One such enzyme is 2-hydroxyacyl-CoA lyase/synthase (HACL/S), which catalyzes the reversible cleavage of 2-hydroxyacyl-CoA (2hcCoA) into formyl-CoA (fCoA) and an aldehyde or ketone. Originally identified in the mammalian α-oxidation pathway of 3-methyl-branched fatty acids, HACL/S has demonstrated remarkable catalytic reversibility, as it is capable of condensing fCoA with various substrates covering a wide range of aldehydes and ketones with different carbon chain lengths. All the enzymes are tetramers, specifically dimers of dimers (α2), where α2 dimer represents a catalytical unit. The three domains have specific functions: the N-terminal domain binds the pyrimidine of ThDP (PYR), the middle domain has a regulatory function (R) and binds ADP, and the C-terminal domain binds the pyrophosphoryl group (PP) of ThDP.

Of particular interest here are the structures of ApbHACL/S with fCoA and D-/L-lCoA. In the structure of ApbHACL/S incubated with fCoA, we trapped a covalent intermediate corresponding to ThDP-hmCoA. This adduct is a product of deprotonated ThDP reacting with fCoA. In these two structures ApbHACACL/S-CoA and ApbHACL/S-fCoA, the distances between C2 of ThDP and C1 of hmCoA are significantly longer than a regular C–C bond (1.54 Å) with 1.8 and 1.9 Å, respectively. Additionally, the C1-O distance in ApbHACL/S-CoA is 1.4 Å which is close to that of a regular hydroxymethyl but 2.0 Å for the same distance in ApbHACL/S-fCoA is much elongated. This suggests that these two intermediates found in these structures represent slightly different reaction states. Similarly, hCoA is partly ordered in the structure of TbHACL/S. Remarkably, in the structure with fCoA there is an intermediate trapped where there is a covalent bond between C2 of ThDP and carbon of hydroxymethyl moiety that is still attached to the sulfur atom of CoA. This seemingly corresponds to the intermediary α−carbanion state with ThDP covalently attached to hmCoA with an elongated C2-C bond distance. Moreover, ApbHACL/S shows the lowest KM (0.41 mM) toward acetaldehyde, which could contribute to successful crystallization with formyl-CoA and acetaldehyde, in addition to lactyl-CoA.

>[4x]SNAMAKSEGKVNGATLMARALQQQGVQYMFGIVGFPVIPIAIAAQREGITYIGMRNEQSASYAAQAASYLTGRPQACLVVSGPGVVHALAGLANAQVNCWPMLLIGGASAIEQNGMGAFQEERQVLLASPLCKYAHQVERPERIPYYVEQAVRSALFGRPGAAYLDMPDDVILGEVEEAAVRPAATVGEPPRSLAPQENIEAALDALQSAKRPLVIVGKGMAWSRAENEVRQFIERTRLPFLATPMGKGVMPDDHPLSVGGARSHALQEADLVFLLGARFNWILHFGLPPRYSKDVRVIQLDLSAEEIGNNRQAEVALVGDGKAIVGQLNQALSSRQWFYPAETPWREAIAAKIAGNQAAVAPMIADNTSPMNYYRVYRDIAARLPRNAIIVGEGANTMDIGRTQMPNFEPRSRLDAGSYGTMGIGLGFAVAAAAVHPGRPVIAVQGDSAFGFSGMEFETAARYGMPIKVIILNNGGIGMGSPAPRDGQPGMPHALSHDARYERIAEAFGGAGFYVTDSAELGPALDAAMAFKGPAIVNIKIAATADRKPQQFNWHG> APTVVHETIRVPAGQTFDGKGQTYVANPNTLGDGSQAENQKPIFRLEAG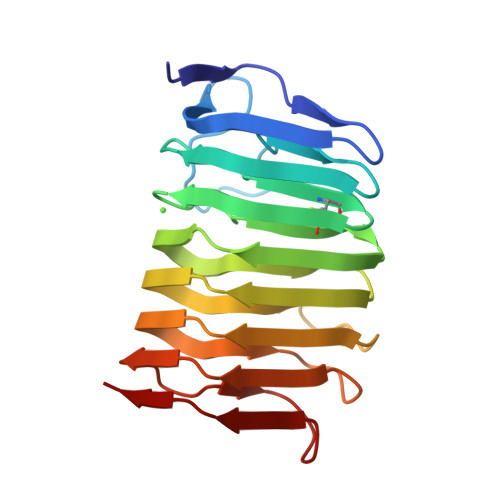ASLKNVVIGAPAADGVHCYGDCTITNVIWEDVGEDALTLKSSGTVNISGGAAYKAYDKVFQINAAGTINIRNFRADDIGKLVRQNGGTTYKVVMNVENCNISRVKDAILRTDSSTSTGRIVNTRYSNVPTLFKGFKSGNTTASGNTQY>[2x]MRLGRIASPDGVAFVSIEGDGPDAVCKEIAEHPFGNPNFTGRSWPLADVRLLAPILASKVIAVGKNYAAHAEEMGGVAPEDPVIFLKPNTAIIGPNVPIQLPADADPVHHEGELAIVIGRPCKDVPAARAAEFILGYTIGNDVSARDQQRKDGQWMRAKGHDTFCPLGPW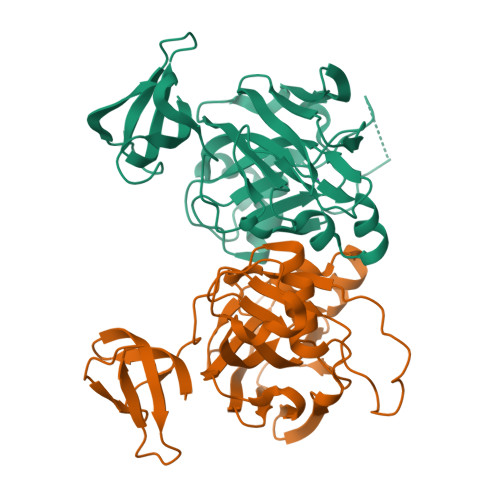IVTDLDPSDVELRTEVNGQVRQRSRTSLLLHDIGRLVEWTSAVMTLLPGDVILTGTPEGVGPIEDGDTVSITVEGIGTLTNPVVRKGKK> MESKVVVPAQGKKITLQNGKLNVPENPIIPYIEGDGIGVDVTPAMLKVVDAAVEKAYKGERKISWMEIYTGEKSTQVYGQDVWLPAETLDLIREYRVAIMGPLTTPVGGGIRSLNVALRQELDLYICLRPVRYYQGTPSPVKHPELTDMVIFRENSEDIYAGIEWKADSADAEKVIKFLREEMGVKKIRFPEHCGIGIKPCSEEGTKRLVRAAIEYAIANDRDSVTLVHKGNIMKFTEGAFKDWGYQLAREEFGGELIDGGPWLKVKNPNTGKEIVIKDVIADAFLQQILLRPAEYDVIACMNLNGDYISDALAAQVGGIGIAPGANIGDECALFEATHGTAPKY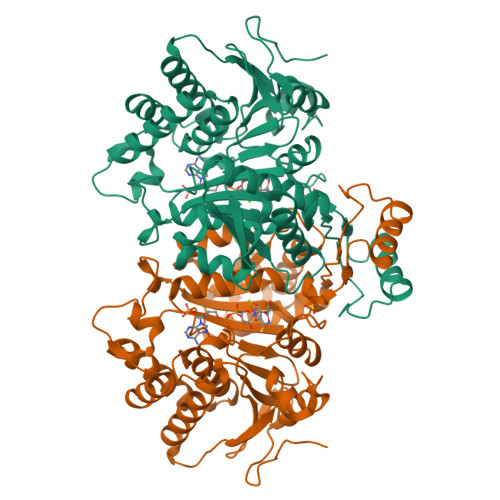AGQDKVNPGSIILSAEMMLRHMGWTEAADLIVKGMEGAINAKTVTYDFERLMDGAKLLKCSEFGDAIIENM> MDNKPETSLDNPVHQRSEPGSETGSSLSTITTHHLTVPPGLTPEEFQELSSSIAEFHSYRINPGQCSSLLAQRIHAPVETVWTVVRRFDKPQTYKHFIKSCSVGEDFRMTVGSTRDVTVISGLPAATSTERLDILDDDRHVTGFSIIGGEHRLRNYRSVTTVHGFERDGEIWTVVLESYVVDVPEGNTEEDTRLFADTVVKLNLQKLASVTETLAREAGNGSVNSRDASHRS

The binding of the plant phytohormone Abscisic acid (ABA) to the family of ABA receptors (PYR/PYL/RCAR) triggers plant responses to abiotic stress. In the resting state, the PYR/PYL receptors are monomers or dimers and display a wide empty ABA binding cavity flanked by two highly conserved loops, named as gate loop and latch loop. To investigate this issue, we have selected as a model SlPYL1 which is a tomato dimeric receptor with known structure that is involved in the induction of stress responsive genes and drought tolerance. Interestingly, the analysis of the structure of SlPYL1 shows that Glu 151 is not involved in the dimerization interface or interacting with ABA; rather, it is located in the latch loop.

Attempts to reproduce the crystallization conditions yielding to a niacin complex with the WT protein were unsuccessful, hence we grew crystals of SlPYL1 with a solution containing 1.0 mM niacin and solved the crystal structure to investigate the role of Glu to Asp 151 substitution in the loop conformation. Our data show that the WT protein interacts solely with a molecule of niacin at ABA carboxylate site which is interacting with NZ of Lys 88. Our crystallographic data shows that the interaction of niacin at the ABA carboxylate site both in the native and in the mutant protein, would compete with ABA for the binding site and might provide the basis for a universal ABA antagonist molecule. To investigate whether the antagonistic effect of niacin was mediated by the binding of the compound to the carboxylate site or to the latch loop of the receptor, we examined the ability of niacin to reverse ABA mediated PP2C inhibition using WT and mutant SlPYL1. Conversely, no effect was observed when assaying the WT protein. Our data showed that while niacin is able to reverse ABA mediated HAB1 phosphatase inhibition using SlPYL1 E151D, it does not display any effect in presence of WT protein.> HGYVSSIQANGQTYPGADPHNPNPESPGWQAENTDLGFVEPSAFSTPAIACHKNARAPPAHATVQAGSTIKLTWNTWPESHHGPVLDYIAPCNGDCSSASAGSLNFVKIAEKGLISGSNPGFWAADELIQNGNSWEVTIPANLAPGKYVLRHEIIALHSAGNPNGAQAYPQCINLEVTGGGSATPSGQPATSFYSPNDPGILFNLYQSFDSYPIP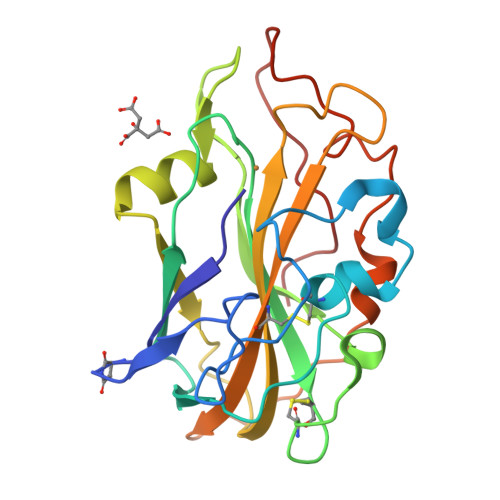GPAVWSG> VLFQGPPTKKVLDENGQSINGKSVLPNATLDYVAKQNFSQYKGIKASAEAIAKGFAFVDQPNEALAELTVKSIKASNGDDVSSLLEMRHVLSKDTLDQK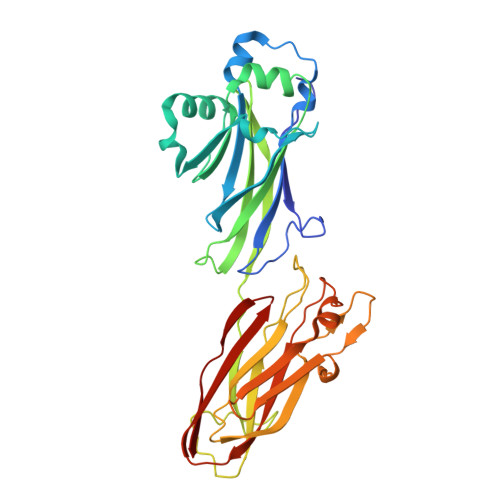LQSLIKEAGISPVGEFYMWTAKDPQAFYKAYVQKGLDITYNLSFKVKKEFTKGQIKNGVAQIDFGNGYTGNIVVNDLTTPEVHKDVLDKEDGKSINNDTVKLGDEVTYKLEGWVVPANRGYDLFEYKFVDHLQHTHDLYLKDKVVAKVAITLKDGTVIPKGTNLVQYTETVYNKETGRYELAFKADFLAQVSRSSAFGADDFIVVKRIKAGDVYNTADFFVNGNKVKTETVVTHT>[2x]AKVIFVLAMDVSGKIASSVESWSSFEDRKNFRKITTEIGNVVMGRITFEEIGRPLPERLNVVLTRRPKTSNNPSLVFFNGSPADVVKFLEGKGYERVAVIGGKTVFTEFLREKL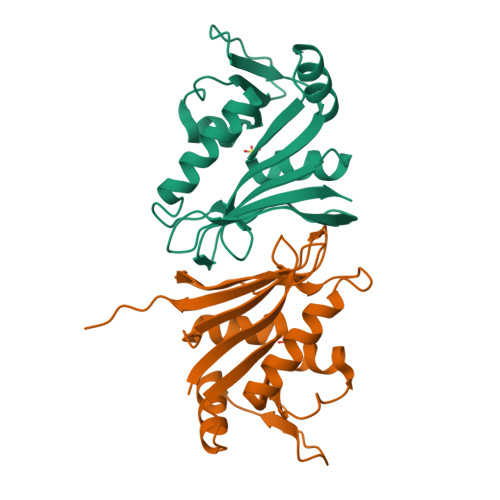VDELFVTVEPYVFGKGIPFFDEFEGYFPLKLLEMRRLNERGTLFLKYSVEKSHR>[4x]M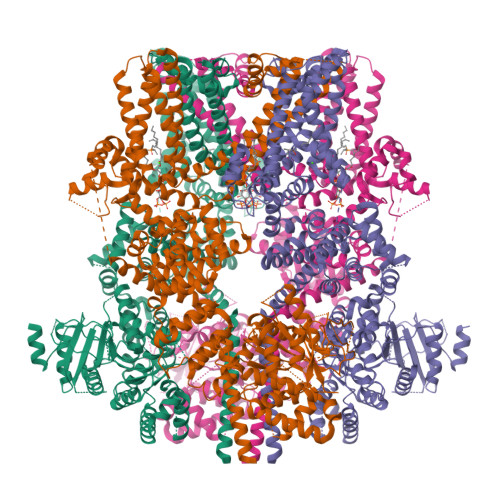ASFEGARLSMRSRRNGTMGSTRTLYSSVSRSTDVSYSDSDLVNFIQANFKKRECVFFTRDSKAMENICKCGYAQSQHIEGTQINQNEKWNYKKHTKEFPTDAFGDIQFETLGKKGKYLRLSCDTDSETLYELLTQHWHLKTPNLVISVTGGAKNFALKPRMRKIFSRLIYIAQSKGAWILTGGTHYGLMKYIGEVVRDNTISRNSEENIVAIGIAAWGMVSNRDTLIRSCDDEGHFSAQYIMDDFTRDPLYILDNNHTHLLLVDNGCHGHPTVEAKLRNQLEKYISERTSQDSNYGGKIPIVCFAQGGGRETLKAINTSVKSKIPCVVVEGSGQIADVIASLVEVEDVLTSSMVKEKLVRFLPRTVSRLPEEEIESWIKWLKEILESSHLLTVIKMEEAGDEIVSNAISYALYKAFSTNEQDKDNWNGQLKLLLEWNQLDLASDEIFTNDRRWESADLQEVMFTALIKDRPKFVRLFLENGLNLQKFLTNEVLTELFSTHFSTLVYRNLQIAKNSYNDALLTFVWKLVANFRRSFWKEDRSSREDLDVELHDASLTTRHPLQALFIWAILQNKKELSKVIWEQTKGCTLAALGASKLLKTLAKVKNDINAAGESEELANEYETRAVELFTECYSNDEDLAEQLLVYSCEAWGGSNCLELAVEATDQHFIAQPGVQNFLSKQWYGEISRDTKNWKIILCLFIIPLVGCGLVSFRKKPIDKHKKLLWYYVAFFTSPFVVFSWNVVFYIAFLLLFAYVLLMDFHSVPHTPELILYALVFVLFCDEVRQWYMNGVNYFTDLWNVMDTLGLFYFIAGIVFRLHSSNKSSLYSGRVIFCLDYIIFTLRLIHIFTVSRNLGPKIIMLQRMLIDVFFFLFLFAVWMVAFGVARQGILRQNEQRWRWIFRSVIYEPYLAMFGQVPSDVDSTTYDFSHCTFSGNESKPLCVELDEHNLPRFPEWITIPLVCIYMLSTNILLVNLLVAMFGYTVGIVQENNDQVWKFQRYFLVQEYCNRLNIPFPFVVFAYFYMVVKKCFKCCCKEKNMESNACCFRNEDNETLAWEGVMKENYLVKINTKANDNSEEMRHRFRQLDSKLNDLKSLLKEIANNIKSNSLEVLFQGPDYKDDDDKAHHHHHHHHHH> GFTSDYSKYLD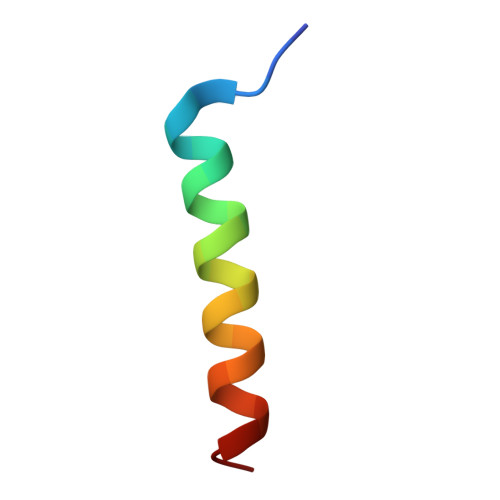SRRAQDFVQWLMNT>[2x]MGSSHHHHHHSSGLVPRGSGAVSGSVQASDRLMKELRDIYRSQSYKTGIYSVELINDSLYDWHVKLQKVDPDSPLHSDLQILKEKEGIEYIL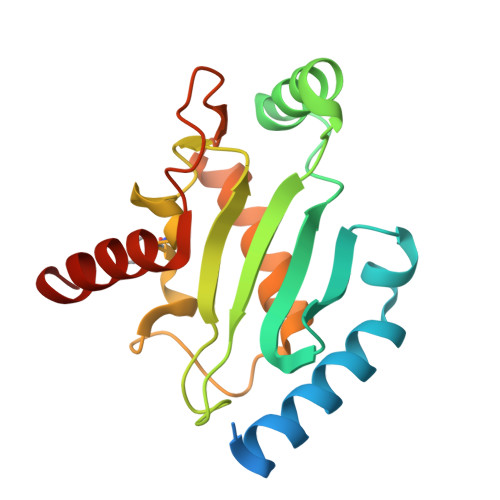LNFSFKDNFPFDPPFVRVVLPVLSGGYVLGGGALCMELLTKQGWSSAYSIESVIMQINATLVKGKARVQFGANKNQYNLARAQQSYNSIVQIHE> MALETWDANSTPATLNTAWPEATDPLNKGDDHIRLLKTVVVN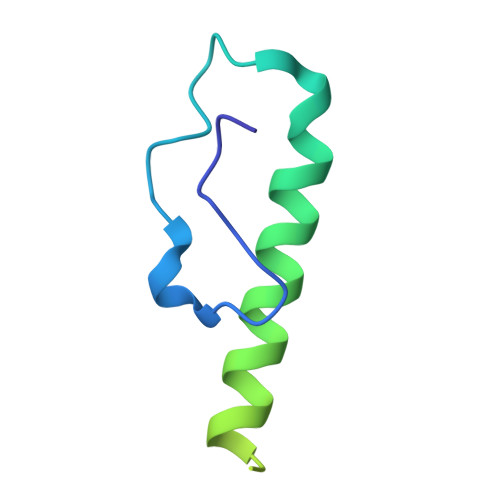FWNKVFDGSKLKTAVVPAAVNSATAGSGFGGFRYQVVNNSDGTKTLRLFTS>AVINTFDGVADYLIRYKRLPDNYITKSQASALGWVASKGNLAAVAPGKSIGGDVFSNREGRLPSASGRTWREADINYVSGARNADRLVYSSDWLIYKTTDHYATFTRI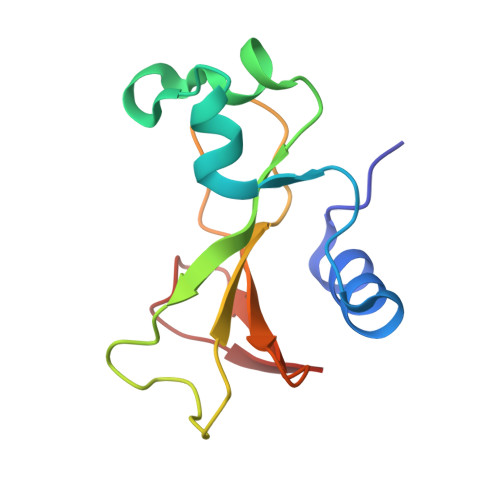R[4x]> SNAGGSATGTGLVYVDAFTRFHCLWDASHPECPARVSTVMEMLETEGLLGRCVQVEARAVTEDELLLVHTKEYVELMKSTQNMTEEELKTLAEKYDSVYLHPGFFSSACLSVGSVLQLVDKVMTSQLRNGFSINRPPGHHAQADKMNGFCMFNNLAIAARYAQKRHRVQRVLIVDWDVHHGQGIQYIFEEDPSVLYFSVHRYEDGSFWPHLKESDSSSVGSGAGQGYNINLPWNKVGMESGDYITAFQQLLLPVAYEFQPQLVLVAAGFDAVIGDPLGGMQVSPECFSILTHMLKGVAQGRLVLA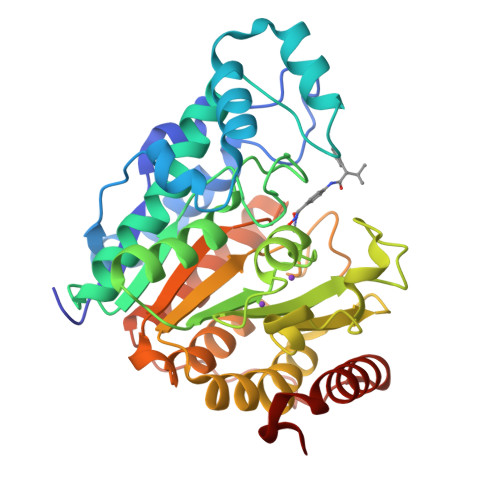LEGGYNLQSTAEGVCASMRSLLGDPCPHLPSSGAPCESALKSISKTISDLYPFWKSLQTFE>[4x]MAAAVVLAAGLRAARRAVAATGVRGGQVRGAAGVTDGNEVAKAQQATPGGAAPTIFSRILDKSLPADILYEDQQCLVFRDVAPQAPVHFLVIP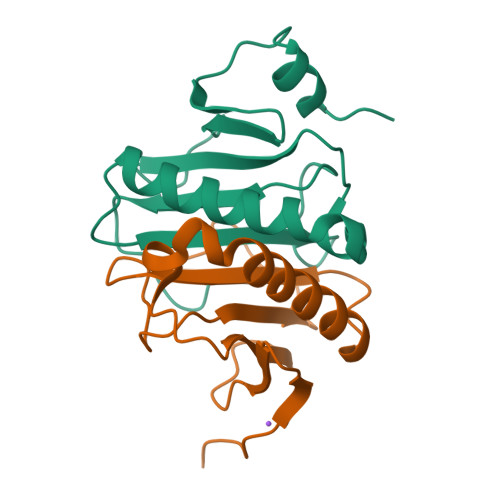KKPIPRISQAEEEDQQLLGHLLLVAKQTAKAEGLGDGYRLVINDGKLGAQSVYHLHIHVLGGRQLQWPPG>MHHHHHHAIGYVWNTLYGWVDTGTGSLAAANLTARMQPISHHLAHPDTKRRFHELVCASGQIEHLTPIAAVAATDADILRAHSAAHLENMKRVSNLPTGGDTGDGITMMGNGGLEIARLSAG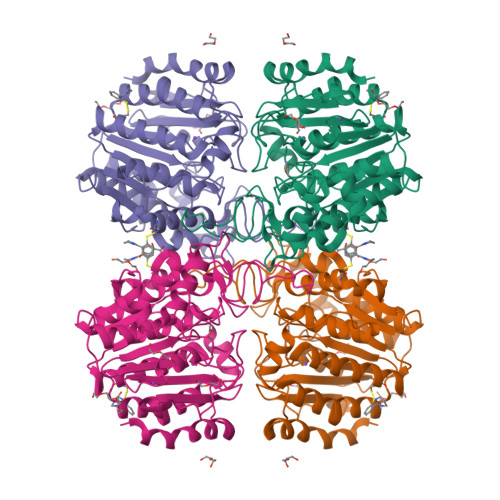GAVELTRRVATGELSAGYALVNPPGHHAPHNAAMGFCIFNNTSVAAGYARAVLGMERVAILDWDVHHGNGTQDIWWNDPSVLTISLHQHLCFPPDSGYSTERGAGNGHGYNINVPLPPGSGNAAYLHAMDQVVLPALRAYRPQLIIVGSGFDASMLDPLARMMVTADGFRQMARRTIDCAADICDGRIVFVQEGGYSPHYLPFCGLAVIEELTGVRSLPDPYHEFLAGMGGNTLLDAERAAIEEIVPLLADIR[2x]>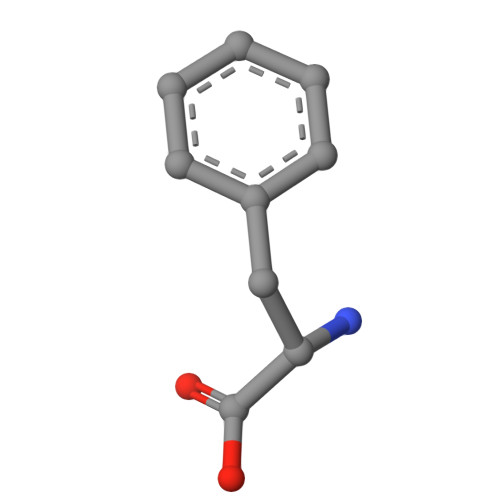 EDF>GPLTEIEHLVQSVCKSYRETCQLRLEDLLRQRSNIFSREEVTGYQRKSMWEMWERCAHHLTEAIQYVVEFAKRLSGFMELCQNDQIVLLKAGAMEVVLVRMCRAYNADNRTVFFEGKYGGMELFRALGCSE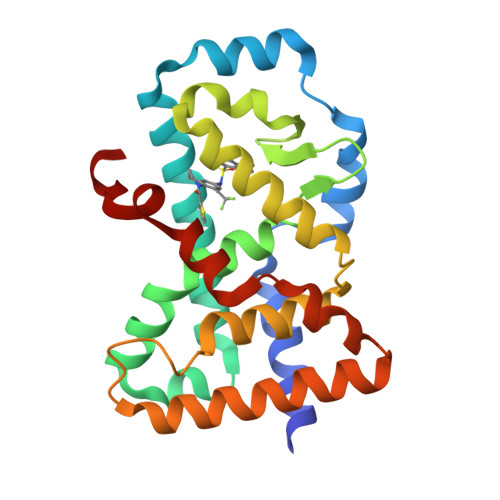LISSIFDFSHSLSALHFSEDEIALYTALVLINAHRPGLQEKRKVEQLQYNLELAFHHHLCKTHRQSILAKLPPKGKLRSLCSQHVERLQIFQ[2x]> PISPIETVPVKLKPGMDGPKVKQWPLTEEKIKALVEICTELEKEGKISKIGPENPYNTPVFAIKKKNSTRWRKLVDFRELNKRTQDFWEVQLGIPHPAGLKKKKSVTVLDVGDAYFSVPLDEDFRKYTAFTIPSINNETPGIRYQYNVLPQGWKGSPAIFQSSMTKILEPFRKQNPDIVIYQYVDDLYVGSDLEIGQHRTKIEELRQHLLRWGLYTPDKKHQKEPPFLWMGYELHPDKWTVQPIVLPEKDSWTVNDIQKLVGKLNWASQIYPGIKVRQLCKLLRGTKALTEVIPLTEEAELELAENREILKEPVHGVYYDPSKDLIAEIQKQGQGQWTYQIYQEPFKNLKTGKYARMRGAHTNDVKQLTEAVQKITTESIVIWGKTPKFKLPIQKETWETWWTEYWQATWIPEWEFVNTPPLVKLWYQLEKEPIVGAETFYVDGAANRETKLGKAGYVTNRGRQKVVTLTDTTNQKTELQAIYLALQDSGLEVNIVTDSQYALGIIQAQPDQSESELVNQIIEQLIKKEKVYLAWVPAHKGIGGNEQVDKLVSAGIRKVL;> PISPIETVPVKLKPGMDGPKVKQWPLTEEKIKALVEICTELEKEGKISKIGPENPYNTPVFAIKKKNSTRWRKLVDFRELNKRTQDFWEVQLGIPHPAGLKKKKSVTVLDVGDAYFSVPLDEDFRKYTAFTIPSINNETPGIRYQYNVLPQGWKGSPAIFQSSMTKILEPFRKQNPDIVIYQYVDDLYVGSDLEIGQHRTKIEELRQHLLRWGLYTPDKKHQKEPPFLWMGYELHPDKWTVQPIVLPEKDSWTVNDIQKLVGKLNWASQIYPGIKVRQLCKLLRGTKALTEVIPLTEEAELELAENREILKEPVHGVYYDPSKDLIAEIQKQGQGQWTYQIYQEPFKNLKT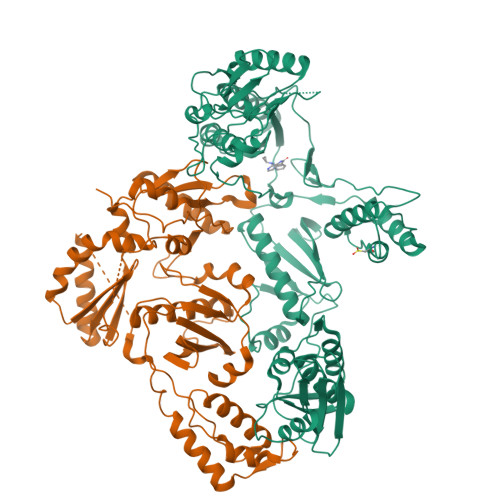GKYARMRGAHTNDVKQLTEAVQKITTESIVIWGKTPKFKLPIQKETWETWWTEYWQATWIPEWEFVNTPPLVKLWYQLEKEPIVGAETF> SMRKKIFKPEELRQALMPTLEALYRQDPESLPFRQPVDPQLLGIPDYFDIVKNPMDLSTIKRKLDTGQYQEPWQYVDDVWLMFNNAWLYNRKTSRVYKFCSKLAEVFEQEIDPVMQSLG

Many proteins, including the EP300/CBP histone acetyltransferases (HATs), contain several targetable domains. EP300 and CBP broadly regulate the activity of other proteins through their protein acetyltransferase catalytic activity. These proteins contain several highly homologous domains, including KIX, bromodomains (BRDs) and HAT domains, through which they interact with, dock to, and acetylate target proteins, respectively. EP300/CBP are critical gene-regulatory targets in cancer, with existing high potency inhibitors of either the catalytic HAT domain or protein-binding bromodomain (BRD). Using crystallography, we identify the binding mechanism of the EP300/CBP-specific BRD inhibitor CCS1477 in complex with the EP300, CBP and BRD4 BRDs, and define components of the CCS1477 catalytic binding core that are required for compound activity.

Since recombinant CBP BRD was more robust in biochemical assays and crystallization studies, Kd values were determined for all compound-CBP interactions by MST, and co-crystal structures of the CBP BRD with five of the seven analogues were determined. Introduction of a butyl group in meta position of the phenyl (compound 6) did not change the binding affinity relative to 5, and the cocrystal structure with CBP showed that R1173 establishes the same Pi-cation and hydrogen-bonding interactions as seen with CCS1477. Among the analogues tested, only compound 6 maintained high activity against CBP but was considerably less potent against BRD4, indicating an increase in target selectivity. While none of the analogues were superior to CCS1477 in terms of binding affinity, substitutions were well tolerated if productive interactions with R1173 were maintained.> SCREKTELTPDQQTLLHFIMDSYNKQRMPQEITNKILKEEFSAEENFLILTEMATNHVQVLVEFTKKLPGFQTL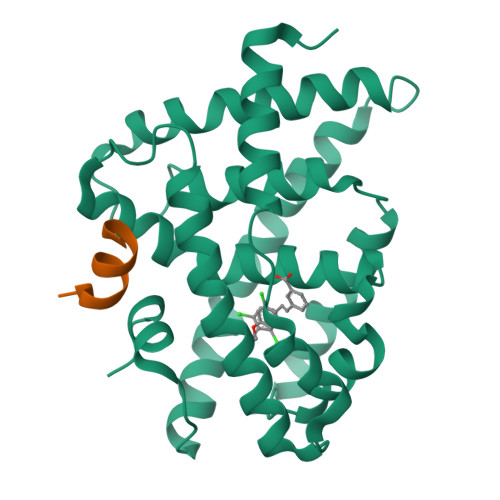DHEDQIALLKGSAVEAMFLRSAEIFNKKLPSGHSDLLEERIRNSGISDEYITPMFSFYKSIGELKMTQEEYALLTAIVILSPDRQYIKDREAVEKLQEPLLDVLQKLCKIHQPENPQHFACLLGRLTELRTFNHHHAEMLMSWRVNDHKFTPLLCEIWDVQ;> KESKDHQLLRYLLDKDEKDLR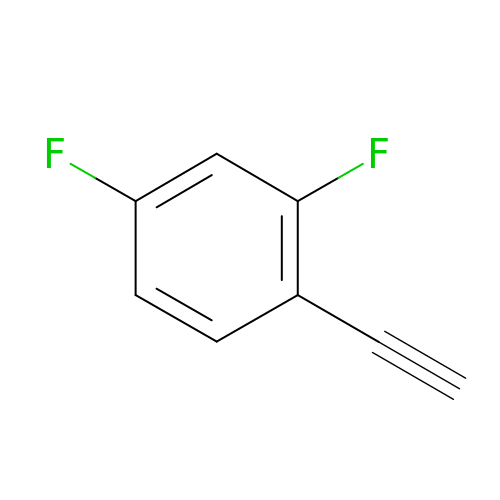1-ethynyl-2,4-difluorobenzene | C8 H4 F2 | HRUJQXRGWQWYDH-UHFFFAOYSA-N>[4x]MRILVTNDDGIYSPGLWALAEAASQF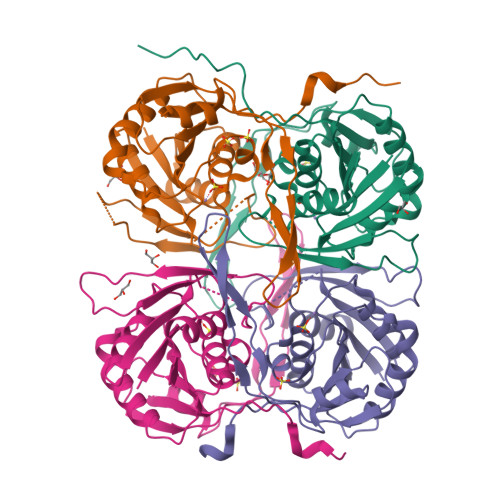GEVFVAAPDTAQSAAGHAITIAHPVRAYPHPSPLHAPHFPAYRVRGTPADCVALGLHLFGPVDLVLSGVNLGSNLGHEIWHSGTVAAAKQGYLFGLSAAAFSVPLNGEVPDFAGLRPWLLRTLETLLRLERPFLVNVNLPLRPKGFLWTRQSVRAYEGVVIPGEDPMGRPFYWFAPRPLKEAEEGTDRWAVAQGFVSATPLRLDLTDETRLQPTLAHD The T=3 icosahedral calicivirus capsid is composed of 180 copies of VP1 with a molecular weight of ~58 kDa, which is divided into the N-terminus (N), the shell (S) and the C-terminal protruding (P) domain (1–5). The S domain forms a shell around the viral RNA genome, while the P domains form protrusions emanating from the shell comprising A/B and C/C dimers. The P domain is further subdivided into P1 and P2 subdomains, with the latter containing the binding sites for cellular receptors and neutralizing antibodies. At conditions found in the gut (i.e., low pH with high metal ion and bile salt concentrations), the P domain rotates and drops onto the shell with intra P domain changes that enhance receptor interactions while blocking antibody binding.

D348E is on the exposed end of the C’D’ loop, far removed from the antibody binding site. Since D348E can escape neutralization by all three monoclonal antibodies, it was expected that, like V339I, the apo structure would also be in the activated conformation in PBS. As with the V339I mutant, the sample used for structural studies was sequenced immediately prior to cryo-EM data collection and verified to contain the mutation. Fig. 8A and B show that, indeed, apo D348E is in the activated state where the P domain is resting on the shell. The loops in apo D348E are in the same conformation as the wt under activating conditions, but far more disordered. Therefore, the D348E allosteric escape mutation activates MNV in a similar manner as V339I. When the aspartate is replaced with a glutamate in the modeled structure, it is too large and collides with T343 and T344. However, in the activated conformation of apo D348E, the D348E side chain rotates up, and there is more than enough space to accommodate the larger side chain. In addition, this orientation places the acidic side chain in an electrostatically favorable location, adjacent to K351 and K345. Therefore, D348E could cause a push/pull structural change where the clashes caused by the mutation push the C’D’ loop out of the wt apo conformation, while simultaneously being pulled toward the activated state conformation because of favorable electrostatic interactions with adjacent lysine residues. Movement in the C’D’ loop is then anticipated to cause a domino effect in the P domain, leading to closed A’B’ and E’F’ loops at the tip of the P domain, a structural conformation which is resistant to neutralization by all three mAbs.

>RMSDGAAPKANGSEASGQDLVPAAVEQAVPIQPVAGAALAAPAAGQINQIDPWIFQNFVQCPLGEFSISPRNTPGEILFDLALGPGLNPYLAHLSAMYTGWVGNMEVQLVLAGNAFTAGKVVVALVPPYFPKGSLTTAQITCFPHVMCDVRTLEPIQLPLLDVRRVLWHATQDQEESMRLVCMLYTPLRTNSPGDESFVVSGRLLSKPAADFNFVYLTPPIERTIYRMVDLPVIQPRLCTHARWPAPVYGLLVDPSLPSNPQWQNGRVHVDGTLLGTTPISGSWVSCFAAEAAYEFQSGTGEVATFTLIEQDGSAYVPGDRAAPLGYPDFSGQLEIEVQTETTKTGEKLKVTTFEMILGPTTNADQAPYQGRVFASVTAAASLDLVDGRVRAVPRSIYGFQDTIPEYNDGLLVPLAPPIGPFLPGEVLLRFRTYMRQIDTADAAAEAIDCALPQEFVSWFASNAFTVQSEALLLRYRNTLTGQLLFECKLYNEGYIALSYSGSGPLTFPTDGIFEVVSWVPRLYQLASVGSLATGRMLKQ[3x]> DDKMDYDFKVKLSSERERVEDLFEYEGCKVGRGTYGHVYKAKRKDGKDDKDYALKQIEGTGISMSACREIALLRELKHPNVISLQKVFLSHADRKVWLLFDYAEHDLWHIIKFHRASKANKKPVQLPRGMVKSLLYQILDGIHYLHANWVLHRDLKPANILVMGEGPERGRVKIADMGFARLFNSPLKPLADLDPVVVTFWYRAPELLLGARHYTKAIDIWAIGCIFAELLTSEPIFHCRQEDIKTSNPYHHDQLDRIFNVMGFPADKDWEDIKKMPEHSTLMKDFRRNTYTNCSLIKYMEKHKVKPDSKAFHLLQKLLTMDPIKRITSEQAMQDPYFLEDPLPTSDVFAGCQIPYPKREFLTEEEPDDKGDKKNQQQ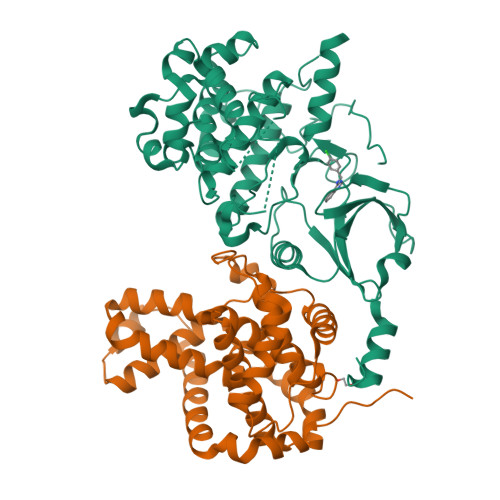QQGNNHTNGTGHPGNQDSSHTQGPPLKKV;> DKAMAGNFWQSSHYLQWILDKQDLLKERQKDLKFLSEEEYWKLQIFFTNVIQALGEHLKLRQQVIATATVYFKRFYARYSLKSIDPVLMAPTCVFLASKVEEFGVVSNTRLIAAATSVLKTRFSYAFPKEFPYRMNHILECEFYLLELMDCCLIVYHPYRPLLQYVQDMGQEDMLLPLAWRIVNDTYRTDLCLLYPPFMIALACLHVACVVQQKDARQWFAELSVDMEKILEIIRVILKLYEQWKNFDERKEMATILSKMPKPKPPPNSEGEQGPNGSQNSSYSQS> CLLCFTTYSERLRICQMFVGMRSPKLEECEEAFTAAFQGLSDTEINYDERSHLHDTFTQMTHALQE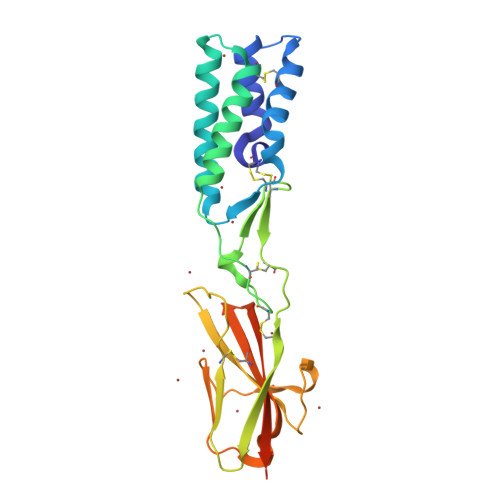LAAAQGSFEVAFPDAAEKMKKVITQLKEAQACIPPCGLQEFARRFLCSGCYSRVCDLPLDCPVQDVTVTRGDQAMFSCIVNFQLPKEEITYSWKFAGGGLRTQDLSYFRDMPRAEGYLARIRPAQLTHRGTFSCVIKQDQRPLARLYFFLNVTGLVPRGSHHHHHHHHHH1,2-DICHLORO-PROPANE | C3 H6 Cl2 | 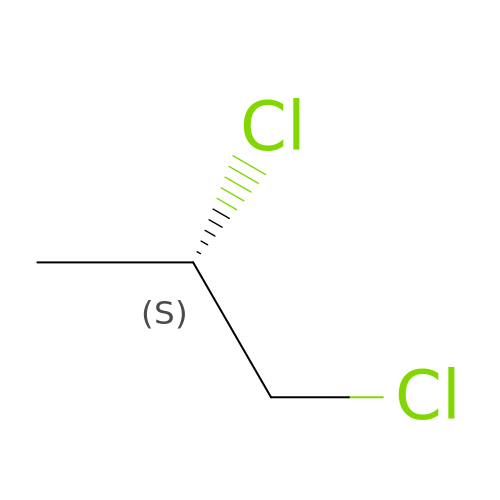KNKRKFALVUDBJE-VKHMYHEASA-N> AVTAAQRIDGGAAFLGDVAIATTKASEHGINVTGRTAEVRVTGGTIRTSGNQAQGLRVGTENAPDNTAVVASVFLQNLIIETSGTGALGVSVHEPQGGGGTRLSMSGTTVRTRGDDSFALQLSGPASATLNDVALETAGQQAPAVVLWQGAQLNAQGLVVQVNGAGVSAIHAQDAGSFTLSGSDITARGLEVVGIYVQEGMQGTLTGTRVTTQGDTAPALQVEDAGTHVSMNGGALSTSGANSPAAWLLAGGSAQFRDTVLRTVGEASHGVDVAAHSEVELAHAQVRADGQGAHGLVVTRSSAMVRAGSLVESTGDGAAALLESGHLTVDGSVVHGHGAAGLEVDGESNVSLLNGARLSSDQPTAIRLIDPRSVLNLDIKDRAQLLGDIAPEAQQPDGSPEQARVRVALADGGTWAGRTDGAVHTVRLLDRGVWTVTGDSRVAEVKLEGGTLAFAPPAQPKGAFKTLVATQGISGTGTIVMNAHLPSGTADVLVAPQGFGDRQVLVVNNTDDGTESGATKVPLIEDEQGHTAFTLGNMGGRVDAGARQYELTASEAQADKARTWQLTPTNELSTTATAAVNAMAIAASQRIWQAEMDVLLRHMSGLHSIGSPGGFWARGLSQRQRLDTGYGPWQKQTVSGIELGLDRRVAGGATTAWSVGMLAGYSETRRDGGAYRAGHVHSAHVGAYVSYLNDSGSYVDGVVKYNRFRHGFDIRTTDLKRVDAKHRSHGLGALLRGGRRIDIDGGWYVEP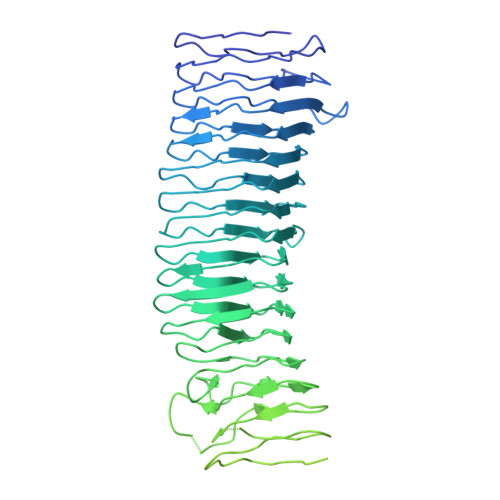QASVAWFHAGGSRYEASNGLRVRADGAHSWVLRAGAEAGRQMRLANGNIVEPYARLGWAQELGADNAVYTNGIRHVTRSRGGFAEARVGVGALLGKRHALYADYEYAKGARFEAPWTLQLGYRYSW>STYDAAAGKATYDASCATCHKTGMMGAPKVGDKAAWAPRIAQGMNTLVSKSIKGYKGTKGMMPAKG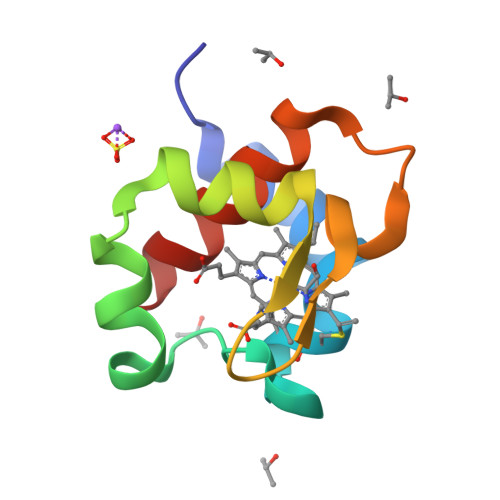GNAKLTDAQVGNAVAYMVGQSK[2x]>GPPAVLLRLSDASGKFEFTEVARGLKVKRNLLDSNDVFV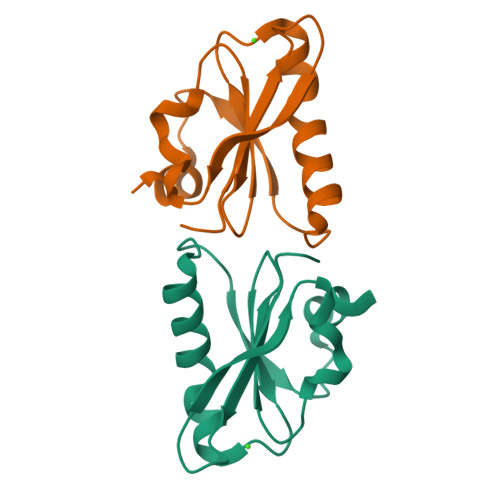LYTGAEVFAWVGKHASVGEKKKALSFAQEYVQKAGLPIHTPVARILEGGENEVFEDFFD[2x]> S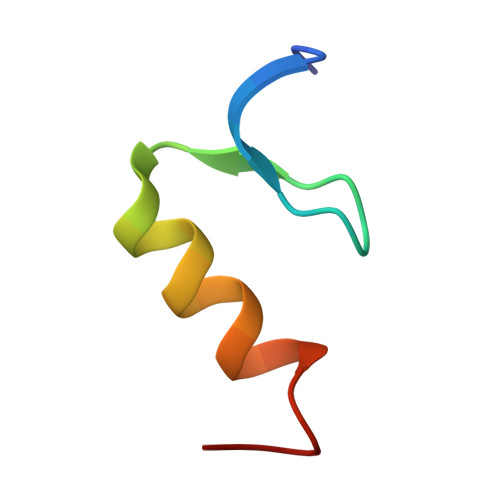SSEGFICPQCMKSLGSADELFKHYEAVHDAGND> GSTQKSLSKEEIERYSRQMIVPGMGKEGQLRLMNAKVLIIGAGGLGCPAAQYLAGAGVGTIGIVDGDSVETSNLHRQVAHATKRVG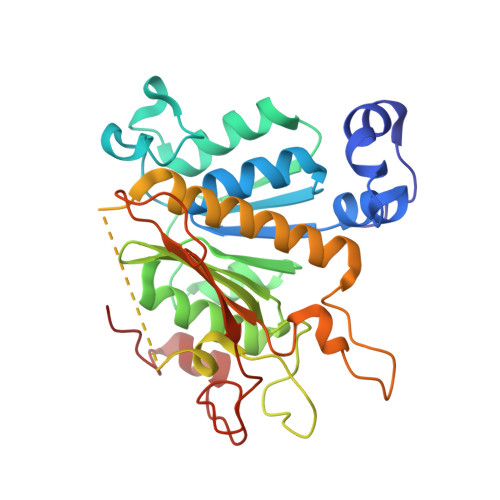MLKVDSLITHLIEINPLPVYVPYRFDLTPQNAAQIIKPWDVILDCTDNPATRYLISDVCVLLGKPLVSAASVQKSGQLIVLNCPPTPQGVVNKKAAPCYRCCFKKPPPPSAQTSCGEAGIMGPVVGMMGVAQAGEAIKILVSQLHMPPKEGEEVSPEKNLVQPTLLIYTYDLNSAIGPYSFRALKMGGRKKDCFACGENSTLTLDGIKSGNPNYVQF>[12x]RMEQSFIMIKPDGVQRGLI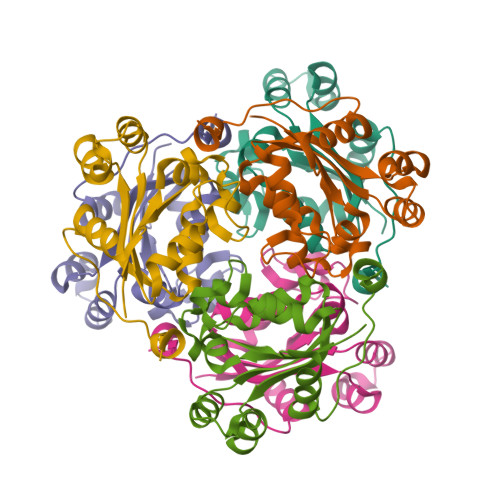GDIISRFEKKGFYLRGMKFMNVERSFAQQHYADLSDKPFFPGLVEYIISGPVVAMVWEGKDVVATGRRIIGATRPWEAAPGTIRADYAVEVGRNVIHGSDSVDNGKKEIALWFPEGLAEWRSNLHPWIYES>[2x]MQLTPTFYDNSCPNVSNIVRDTIVNELRSDPRIAASILRLHFEDCFVNGCDASILLDNTTSFRTEKDAFGNANSARGFPVIDRMKAAVESACPRTVSCADLLTIAAQQSVTLAGGPSWRVPLGRRDSLQAFLDLANANLPAPFFTLPQLKDSFRNVGLNRSSDLVALSGGHTFGKNQCRF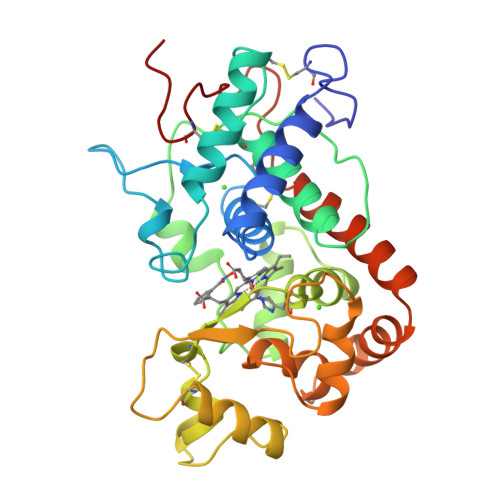IMDRLYNFSNTGLPDPTLNTTYLQTLRGLCPLNGNLSALVDFDLRTPTIFDNKYYVNLEEQKGLIQSDQELFSSPNATDTIPLVRSFANSTQTFFNAFVEAMDRMGNITPLTGTQGQIRLNCRVVNSNS>[2x]GSYAEGQRKRRNTIHEFKKSAKTTLIKIDPALKIKTK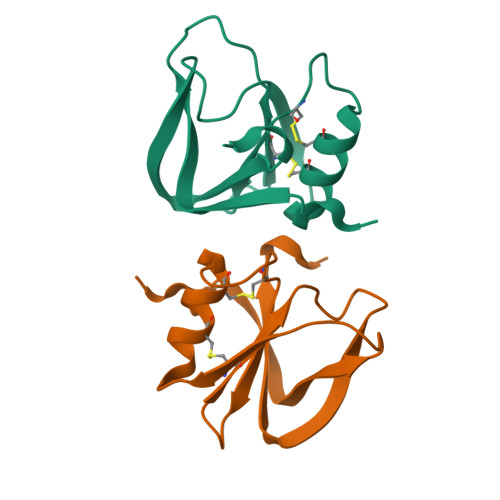KVNTADQCANRCTRNKGLPFTCKAFVFDKARKQCLWFPFNSMSSGVKKEFGHEFDLYENKDYIR>MNTIHH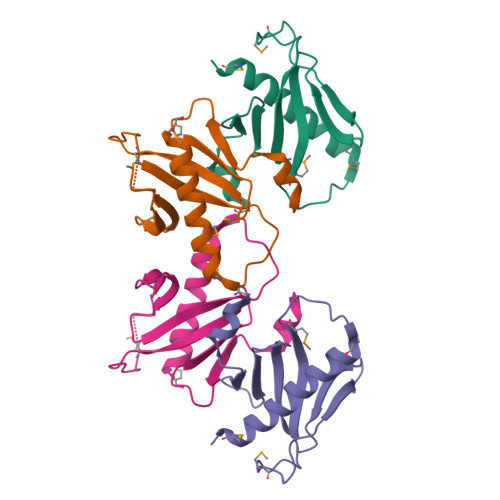HHHNTSGSGGGGGRLVPRGSMSENLYFQGSMSKNNIFNKYPTIIHGEARGENDEFVVHTRYPRFLARKSFDDNFTGEMPAKPVNGELGQIGEPRRLAYDSRLGLWLSDFIMLDNNKPKNMEDWLGQLKAACDRIAADDLMLNEDAADLEGWDD[2x]> MQSLNVNGTLMTYSESGDPHA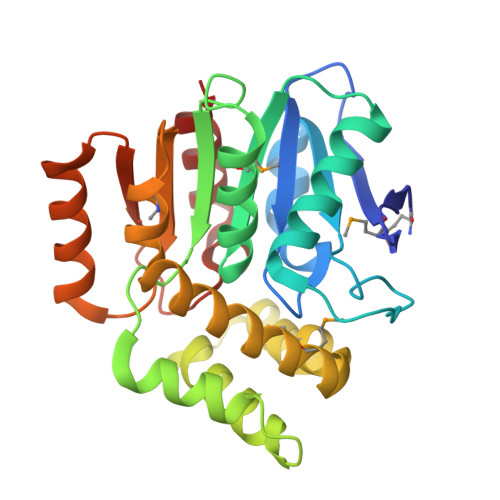PTLFLLSGWCQDHRLFKNLAPLLARDFHVICPDWRGHDAKQTDSGDFDSQTLAQDLLAFIDAKGIRDFQMVSTSHGCWVNIDVCEQLGAARLPKTIIIDWLLQPHPGFWQQLAEGQHPTEYVAGRQSFFDEWAETTDNADVLNHLRNEMPWFHGEMWQRACREIEANYRTWGSPLDRMDSLPQKPEICHIYSQPLSQDYRQLQLEFAAGHSWFHPRHIPGRTHFPSLENPVAVAQAIREFLQA> GMSVAAEVAQVAQSAIDDFNAAYGLCLDDDRLE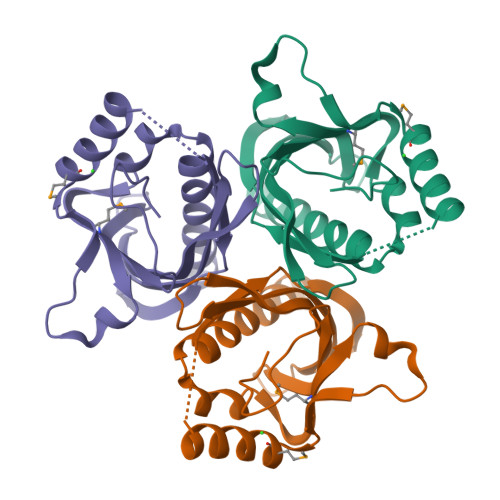QWPTLFVDDCLYQVIARENVDNGLPAAVMYCDSKGMLADRVVALRKANVFPEHFNRHLIGRAVITGVEGDQVSAEASYVVFQTRNDGETRIYNAGKYVDRFDLSGGTVRLKSRTCIYDTLRIATLLATPI>[5x]DYKDDDDKLHSQANLMRLKSDLFNRSPMY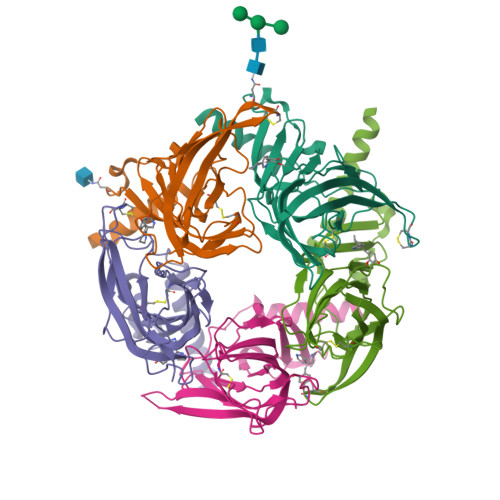PGPTKDDPLTVTLGFTLQDIVKADSSTNEVDLVYYEQQRWKLNSLMWDPNEYGNITDFRTSAADIWTPDITAYSSTRPVQVLSPQIAVVTHDGSVMFIPAQRLSFMCDPTGVDSEEGATCAVKFGSWVYSGFEIDLKTDTDQVDLSSYYASSKYEILSATQTRQVQHYSCCPEPYIDVNLVVKFRERRAGNGFFRNLFD>[60x]MYFFSVDPRNGASKSGDVCGSCCCESISARPGEVNGVMVSYAAWSAPLRGHGLTNKTTFEIDGVSVTPPKVSNAFGRTKVGVVFEGTLSDLFPNPEGEQVEYEISELNGPSNGVVELGANGAFTYTPGALFTGVDRFWFSINGNIGEYVISVDPTTSELPQPPFTTPVYVPAARRSVDPRTHVLKFVLGVSPAAIPGDVYRLTVRQVAIDCDGNEFVHISCYDISIGSCG

Caudovirales, the taxonomic order for the tailed double-stranded DNA bacteriophages, is characterized by the presence of a tail—a host cell attachment organelle that is connected to the genome-containing spherical or elongated capsid via a neck. We describe cryo-EM structures of the neck, the neck-capsid and neck-tail junctions, and capsid of the Agrobacterium phage Milano. The tail to capsid junction involves a symmetry mismatch that is bridged by the neck, and is therefore crucial for the assembly of tailed phage. The extensive network of disulfide bonds within and between neck, collar, capsid and tail provides an exceptional structural stability to Milano.

The 15-fold, 12-fold and 3-fold symmetrized maps of the neck were used to build atomic models of the collar, portal, and neck devoid of capsid (portal + neck 1 + neck 2 + tail terminator + collar), respectively. The Milano collar is made up of four rings of gp13 pentadecamers (15 × gp13). The gp13 subunit contains two β-strand-rich jellyroll-like domains. Domain 1 (residues 1–69, 167–230) forms the wall of the collar, and we thus named it the wall domain (W domain), whereas domain 2 (residues 70–166) decorates the collar wall, and we named it the decorating domain (D domain). DALI search results suggest that the D domain of gp13 is structurally similar to glycan-interacting and cell surface binding proteins. Four collar rings are stacked and stabilized by complementary electrostatic charges on the interacting surfaces of their W domains. The W domain of each gp13 protomer is covalently linked to its neighboring subunits by four disulfide bonds, one with each neighbor within the same ring (Cys23-Cys229) and one with each neighbor along the left-handed 12-start helices (Cys22-Cys211). The collar of Milano is structurally distinct from that of T4 and XM1 bacteriophage. In contrast, the Milano collar consists of four rings (4 x gp13) surrounding the whole neck and displaying no fibers or spike-like structures. An elaborate network of disulfide bonds in the collar suggests that they play a role in the overall robustness of Milano particles against mechanical stress, supported by the observation that this stability is lost under reducing conditions.> FRAIIESPEGAGHVGYQYRRNTGSTMRMVSDVLDERVSLWDFHCDPSGNVIQPGPNVDSRQYLQAAIDYVSSNGGGTITIPAGYTWYLGSYGVGGIAGHSGIIQLRSNVNLNIEGRIHLSPFFDLKPFQVFVGFDNGDPASSGNLENCHIYGHGVVDFGGYEFGASSQLRNGVAFGRSYNCSVTGITFQNGDVTWAITLGWNGYGS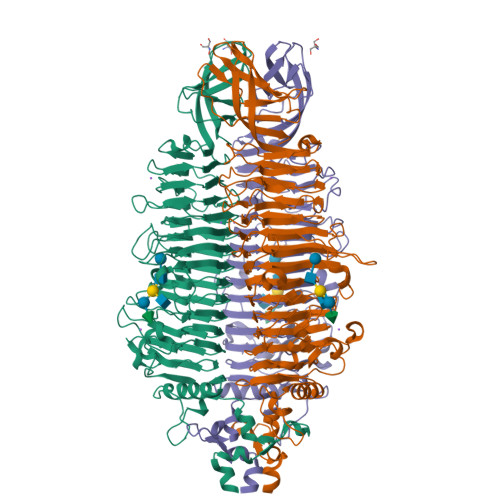NCYVRKCRFINLVNSSVNANHSTVYVNCPYSGVESCYFSMSSSFARNIACSVALHQHDTFYRGSTVNGYCRGAYVVMHAAEAAGAGSYAYNMQVENNIAVIYGQFVILGSDVTATVSGHLNDVIVSGNIVSIGERAAFSAPFGAFIDIGPDNSGASNVQDIQRVLVTGNSFYAPANITDSAAITLRANLNGCTFIANNFDCRYMVYNAPGTTSPVVQNLVWDKSNVIGGTHANQRAGQNLFDMQFASVVNSTIEVQLSCEDLSMFSCILFPASCQLSYSKITVDSAWTKSMSNTAVFEGNQQAGANVYVSYPATVNLTSYNTQGAVPFFSTDTNYAWVTSAYSLSINENLDFSPPATYTNKANGQLVGVGYNEIGGVRSVSVRLMLQRQV> GAMDKRTQPTTGTSGGYYFSFWTDTPNSVTYTNGNGGQFSMQWSGNGNHVGGKGWMPGTSRTIKYSGSYNPNGNSYLAVYGWTRNPLIEYYIVENFGTYNPSSGGQKKGEVNVDGSVYDIYVSTRVNAPSIDGNKTFQQYWSVRRNKR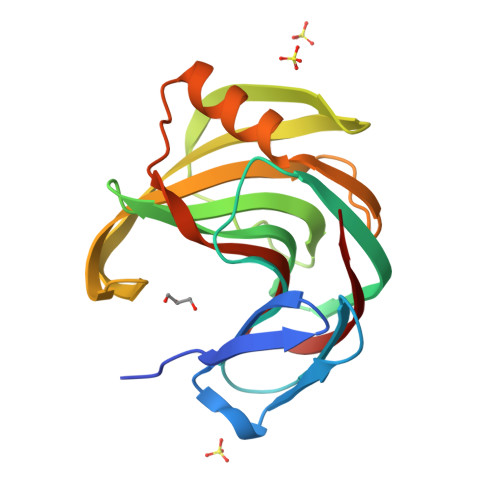SSGSVNTGAHFQAWKNVGLNLGTHDYQILAVEGYYSSGSASMTVSQ Among such receptors is macrophage-inducible C-type lectin (Mincle, gene symbol CLEC4E), a member of the C-type lectin receptor (CLR) family, which functions as an immune sensor for both pathogens and damaged self. Mincle recognizes its ligands via a calcium-dependent sugar-binding site, containing a conserved EPN (Glu-Pro-Asn) motif, and a hydrophobic groove on the carbohydrate recognition domain (CRD), which are in combination the major characteristics of Mincle. In Takifugu rubripes, one of the first vertebrates whose whole genome was completely sequenced, a protein sequence bearing the EPN motif and a hydrophobic groove was found (XP_029706534.1). Altogether, trMincle shares similar characteristics with mammalian Mincle in its amino acid sequence and its FcRγ-dependent cell surface expression.

As trMincle was predicted to be a type II transmembrane protein, we constructed the extracellular domain of trMincle as a soluble recombinant protein followed by column-based purification. The crystal structure of trMincle was determined at 1.7 Å resolution. A calcium ion was coordinated with Glu-Pro-Asn (EPN) and Trp-Asn-Asp (WND), two well-conserved motifs, suggesting the typical sugar-binding pocket observed in other mammalian C-type lectins was also present in trMincle. Furthermore, one glycerol molecule in the media interacted with the EPN motif within the hydrophilic pocket, and hydroxyl groups at C1 and 2 of glycerol formed coordination bonds with calcium ion, which is similar to the reported sugar-binding mode of mammalian Mincle.Fig. 2 trMincle is structurally similar to boMincle. Indeed, overall, both fish and mammalian Mincle possessed hydrophilic pockets and adjacent grooves;, although the amino acid residues were not identical. Moreover, the molecular dynamics simulation suggested that the trMincle CRD can create a typical groove similar to a mammalian Mincle. The crystal structure of trMincle suggests the formation of a stable homodimer.

>[4x]MNGTAEERNKFDKLDPYFQQGWFHFQKSLYYISSVKNTWHLSREYCLQEGADLAIINSRAEQAFLENFKMTLWIGLMEQRSERTWRWVDGTPLTESYWSLGEPNNYEGRQEQCVEQIDREDKKGWNDLVCEFSNFYMCEKRIFP The p190RhoGAP proteins, p190RhoGAP-A (ARHGAP35) and p190RhoGAP-B (ARHGAP5), are key regulators of Rho GTP hydrolysis and are highly important for maintenance of proper Rho signaling. They share over 50% sequence identity and a domain organization containing a GTP-binding GTPase domain, four FF domains and a C-terminal GAP domain. We identify two GTPase-like folds in the middle domain of both p190RhoGAP-A and -B which we term pG1 and pG2, and show that they are important for GAP activity toward RhoA. Thus, we classify p190RhoGAP pG1 and pG2 as psuedoGTPases.

We obtained crystals of the p190RhoGAP-A and p190RhoGAP-B pG1 domains that diffract to 1.9 and 2.6 Å resolution, respectively. The root mean square deviation (r.m.s.d.) between the two pG1 structures is 1.8 Å over 128 Cαs, and 2.7 Å (135 Cαs) between the prototypical small GTPase H-Ras and p190RhoGAP-A pG1. Crystal structures of pG1 reveal similarities to the Ras-like GTPase superfamily. All five G motifs are degraded in p190RhoGAP pG1. In p190RhoGAP, helix α1 (which follows the P-loop) is extended and sterically occludes the phosphate-binding cavity. Switch I (G2) is completely absent in p190RhoGAP pG1 due to an 11-residue deletion. Switch II (G2) is also degraded in p190RhoGAP pG1, and places a glutamate side chain (Glu636) where the γ-phosphate of GTP binds to canonical small GTPases. The G4 and G5 motifs are disordered in our structures, but their sequence divergence suggests degraded ability to bind guanine base, and in our structures the guanosine-binding site appears to be sterically hindered by the side chains of Glu606 and Arg739, which form a predicted salt bridge with one another. Taken together, these studies establish that the isolated pG1 domain of p190RhoGAP is not a nucleotide-binding domain.

> GSSTNIDKVNLFILGKDGLAQELANEIRTQSTDDEYALDGKIYELDLRPVDAKSPYFLSQLWTAAFKPHGCFCVFNSIESLSFIGEFIGKIRTEASQIRKDKYMANLPFTLILANQRDSISKNLPILRHQGQQLANKLQCPFVDVPAGTYPRKFNETQIKQALRGVLESVKHNLDV> MDSRVTAMTTSQLRTWLRDWVLATTGLPAEEITDDKPMQSFGLSSRDVVLLSGELENLLGVKLDA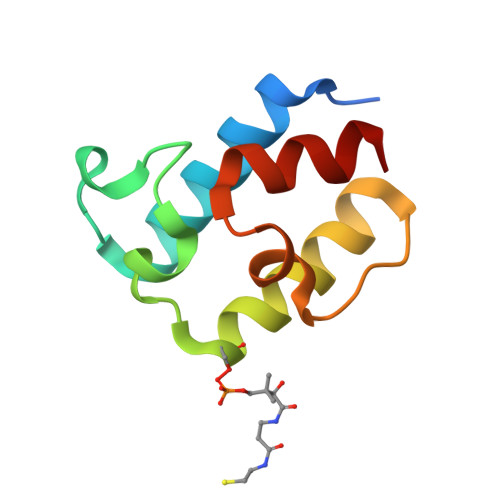TIAYEYPTIAALSQRLIEGA2-(6-morpholin-4-ylpyrimidin-4-yl)-4-(1,2,3-triazol-1-yl)-1~{H}-pyrazol-3-one 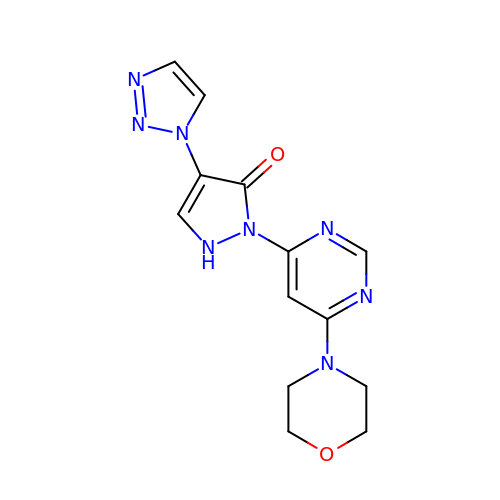| C13 H14 N8 O2 | IJMBOKOTALXLKS-UHFFFAOYSA-N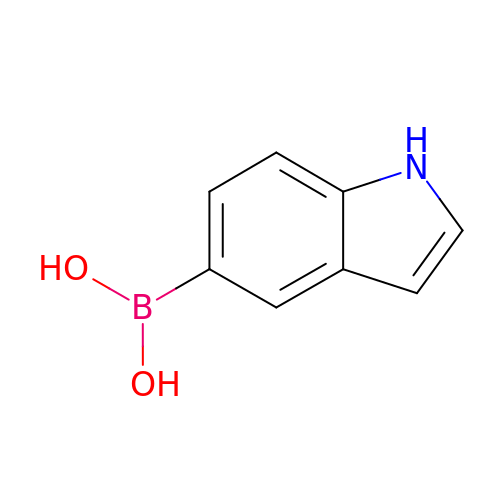1~{H}-indol-5-ylboronic acid | C8 H8 B N O2 | VHADYSUJZAPXOW-UHFFFAOYSA-N> AGWNVNSKQNIAVYWGQNSANSQSTQQRLSFYCNDANINVIDIAFLNGITPPMTNFANAGDRCTPFSDNPWLLQCPEIEADIKTCQANGKTILLSLGGDSYTQGGWSSTGAAQSAADQVWAMFGPVQSGSSVHRPFGSAVVDGFDFDFEATTNNLAAFGAQLKSRTNAAGGKKYYFSAAPQCFFPDAAVGALINAVPMDWIQIQFYNNPCGVSGFTPGTSTQNNYNYQTWENWAKTSPNPNVKLLVGIPAGPGAGRGYVSGSQLTSVFQYSKGFSTFAGAMMWDMSQLYQNTGFETQVVNALR

The endo-chitinase Chit33 from T. harzianum is included in the GH18 family. Chit33 belongs to class III (plant-type) enzymes characterized by the presence of shallow catalytic tunnels and open substrate-binding grooves. Chit33 is folded into a (β/α)8 barrel domain, similarly to family 18 chitinases. The DxDxEx conserved catalytic motif is located at the end of strand β4 of the barrel, with Glu167 being the catalytic acid protonating the glycosidic bond and Asp165 playing a key role in assisting the acetamido group in its nucleophilic attack and stabilizing the developing positive charge on the oxazolinium ion.

To elucidate the molecular basis of its enzymatic activity, the crystal structure of native Chit33 was solved at 1.12 Å resolution. The crystals belong to the P 21 21 21 space group, with one molecule in the asymmetric unit and 50% solvent content within the cell. The structure was determined by means of molecular replacement using the co-ordinates from the Saccharomyces cerevisiae chitinase 1, ScCTS1, as the search model. A short and not well-defined α1, a bent α8, and the presence of two β-strand insertions after β2 are widespread features of other family 18 chitinases. Moreover, the short loops connecting the secondary structure elements are responsible for the definition of a tiny TIM barrel, which diverges from the bacterial-type chitinases embracing large βα loops, which even include a full chitin insertion α/β domain (CID). Furthermore, three disulfide bonds, Cys51-Cys103, Cys81-Cys93 and Cys200-Cys228, are detected in the Chit33 polypeptide chain. In particular, the longer β1α1 loop makes a deeper cavity in Chit33, conferring a more tunnel-like appearance to its active site. A TRIS molecule from the buffer solution was captured at the active site of the native crystals, making polar interactions through its hydroxyl groups with the catalytic Asp165 and Glu167, as well with Gln222 located at the end of β6. As shown in the Chit33-NAG4 complex, Ser118 presents a dual conformation in the free enzyme that is fixed upon ligand binding and orients to make a polar link to O6 from the sugar at subsite −2. Structural comparison of the wild type and the complex with NAG4 Chit33 does not show significant differences, apart from a visible reorganization of the Asp117 and Arg274 side chains that approach the substrate, enabling direct polar links.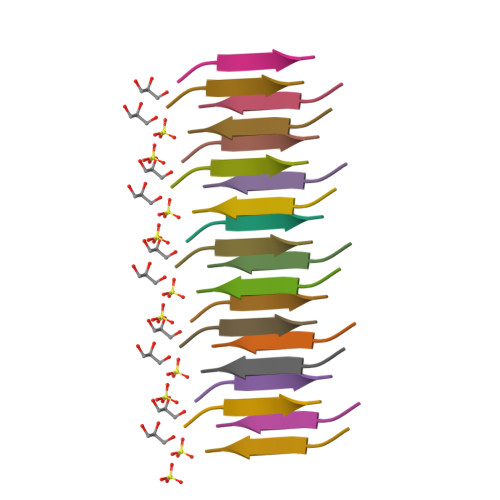>KALGIS[2x]> GAMAAPAACTRFSDNYDIKEELGKGAFSIVKRCVQKSTGFEFAAKIINTKKLTARDFQKLEREARICRKLHHPNIVRLHDSIQEENYHYLVFDLVTGGELFEDIVAREFYSEADASHCIQQILESVNHCHQNGVVHRDLKPENLLLASKAKGAAVKLADFGLAIEVQGDHQAWFGFAGTPGYLSPEVLKKEPYGKSVDIWACGVILYILLVGYPPFWDEDQHRLYSQIKAGAY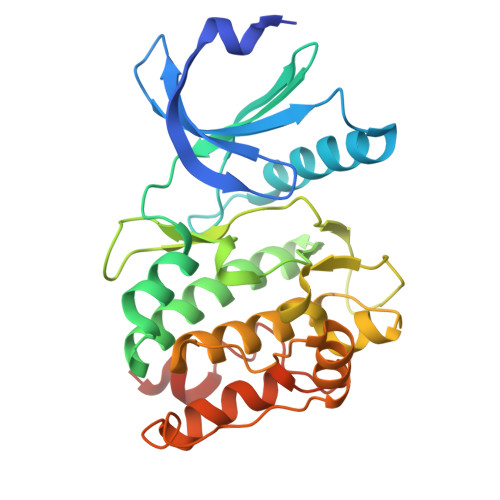DYPSPEWDTVTPEAKNLINQMLTVNPNKRITAAEALKHPWICQRERVASVVH> SHMLRLSAPGQLDDDLCLLGDVQVPVFLLRL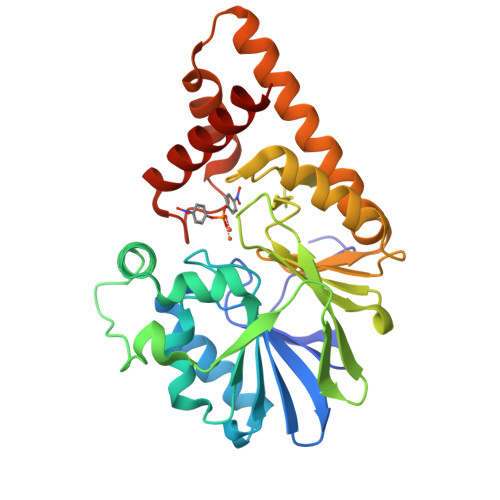GEASWALVEGGISRDAELVWADLCRWVADPSQVHYWLITHKHYDHCGLLPYLCPRLPNVQVLASERTCQAWKSESAVRVVERLNRQLLRAEQRLPEACAWDALPVRAVADGEWLELGPRHRLQVIEAHGHSDDHVVFYDVRRRRLFCGDALGAFDEAEGVWRPLVFDDMEAYLESLERLQRLPTLLQLIPGHGGLLRGRLAADGAESAYTECLRLCRRLLWRQSMGESLDELSEELHRAWGGQSVDFLPGELHLGSMRRMLEILSRQALPLD>[2x]MTVQCKPIPALYTVYVLRSTVRHASLYIGSTPNPPRRLKQHNGLVPGGAARTSRSSLRPWEMVALVSGFPSMVAALKFQWALTNPHLSVHIPSASRLTVATQTKANGRPQRPPRSLASVVANLHLLLRVPSFARWPLRVHFFRRDVFAAWEKWCAAASERLR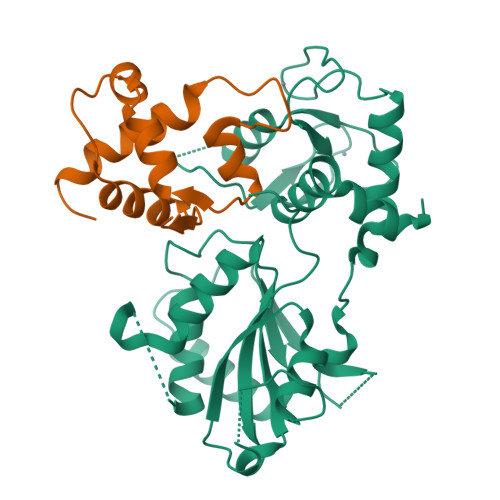PSLAVVTDFEGGSEGLAGAVVGGEEGRERGEGAPCWGIHALPLDYEPIKDYVAKGQEIFEFERQGACVVCREEMASGDGLQALCTNQGCDGVGHLSCWSRHFLKGAEADSILPVQGQCPKCGGEMEWGNMMKELTLRTRGQKEVEKLLKRKRRRATKKTANA;>MEDTETSLVASPTDQQVSLFRYITQAVVTAPRAKDPANPSWHEKMLMYDPIILEDLTAWLNSGQLDRVGYDGEVAPGDVKKWCESKSVCCLWRVSLNGKERKRF[2x]>SNAMVEAIIFDMDGVLFDTEKYYYDRRASFLGQKGISIDHLPPSFFIGGNTKQVWENILRDEYDKWDVSTLQEEYNTYKQNNPLPYKELIFPDVLKVLNEVKSQGLEIGLASSSVKADIFRALEENRLQGFFDIVLSGEEFKESKPNPEIYLTALKQLNV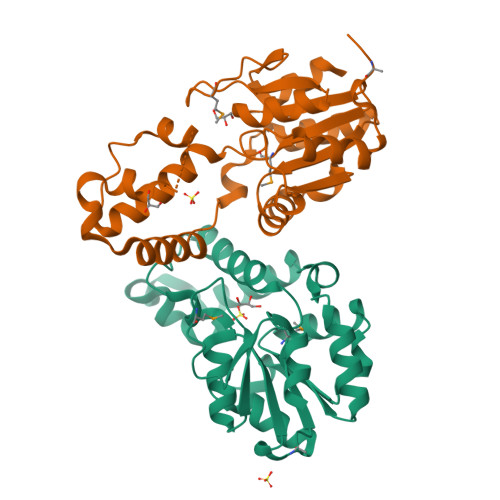QASRALIIEDSEKGIAAGVAADVEVWAIRDNEFGMDQSAAKGLLDSLTDVLDLI[2x]>[12x]MAGKLMHALQYNSYGGGAAGLEHVQVPVPTPKSNEVCLKLEATSLNPVDWKIQKGMIRPFLPRKFPCIPATDVAGEVVEVGSGVKNFKAGDKVVAVLSHLGGGGLAEFAVATEKLTVKRPQEVGAAEAAALPVAGLTALQALTNPAGLKLDGTGKKANILVTAASGGVGHYAVQLAKLANAHVTATCGARNIEFVKSLGADEV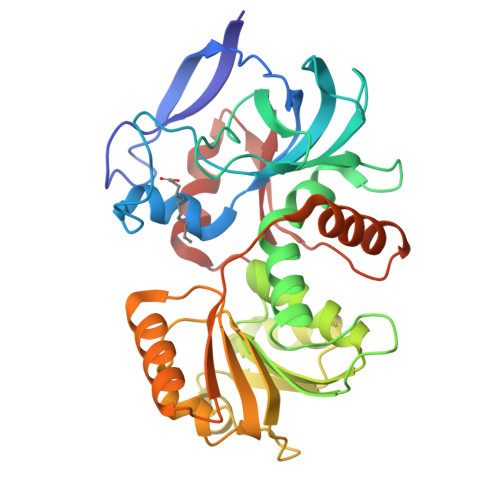LDYKTPEGAALKSPSGKKYDAVVHCANGIPFSVFEPNLSENGKVIDITPGPNAMWTYAVKKITMSKKQLVPLLLIPKAENLEFMVNLVKEGKVKTVIDSKHPLSKAEDAWAKSIDGHATGKIIVEP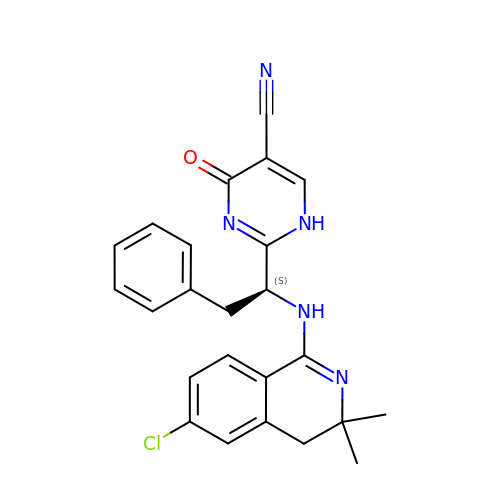2-{(1S)-1-[(6-chloro-3,3-dimethyl-3,4-dihydroisoquinolin-1-yl)amino]-2-phenylethyl}-4-oxo-1,4-dihydropyrimidine-5-carbonitrile | C24 H22 Cl N5 O | SSQLUPVACAMCTQ-FQEVSTJZSA-N>GSLVEEELDPFSLVADELSLLSNKLREMVLAEVPKLASAAEYFFKRGVQGKQFRSTILLLMATALDVRVPEALIGESTDIVTSELRVRQRGIAEITEMIHVASLLHDDVLDDADTRRGVGSLNVVMGNKMSVLAGDFLLSRACGALAALKNTEVVALLATAVEHLVTGETMEITSSTEQRYSMDYYMQKTYYKTASLISNSCKAVAVLTGQTAEVAVLAFEYGRNLGLAFQLIDDILDFTGTSASLGKGSLSDIRHGVITAPILFAMEEFPQLREVVDQVEKDPRNVDIALEYLGKSKGIQRARELAMEHANLAAAAIGSLPETDNED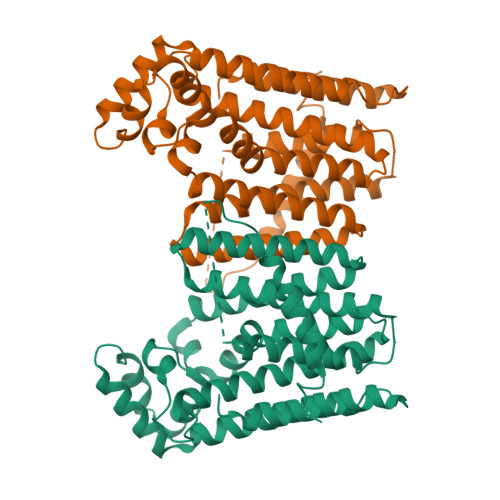VKRSRRALIDLTHRVITRNK[2x]>[6x]MQVVR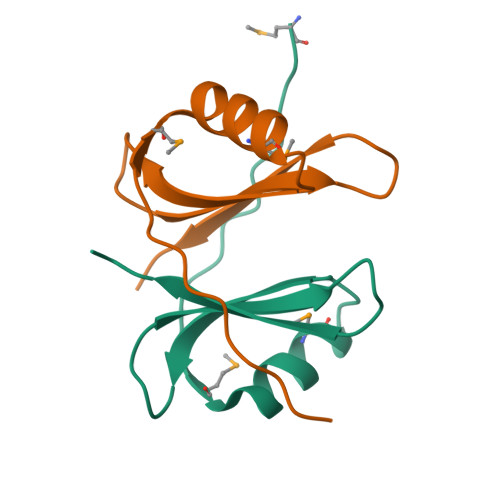TKNVTLKPMDVEEARLQMELLGHDFFIYTDSEDGATNILYRREDGNLGLIEAKLEHHHHHH>[8x]NNLISFTMKRIVLFLILLTKAASANLISFTFKKFNET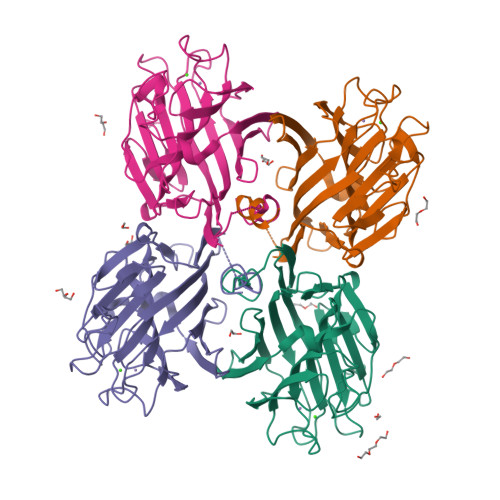NLILQRDATVSSGKLRITKAAENGVPTAGSLGRAFYSTPIQIWDNTTGTVASWATSFTFNLQAPNAASPADGLAFALVPVGSQPKDKGGFLGLFDSKNYASSNQTVAVEFDTFYNGGWDPTERHIGIDVNSIKSIKTTSWDFANGENAEVLITYDSSTNLLVASLVHPSQKTSFIVSERVDLTSVLPEWVSVGFSATTGLSKGYVETNEVLSWSFASKLSINKEDEENKLAIFNLEGKAINNLA> MSNILFKPTHLPISKPFHALLANILSEHQAKSEVQATSKEVVMNFRDSSYSAEDGGFHPVEIALSQSSDGQWCIEYITDFAYVGNHFPELERCLDFDFQRGDFFTAYHGWNPIVGNRDARELYQLWESNFLAYVATEAFDDISLTSA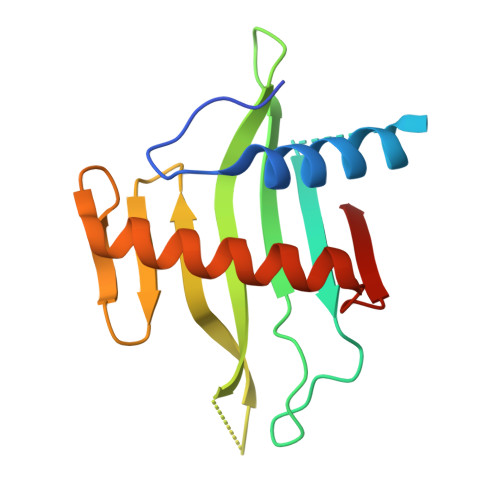P>SMNLIPTVIETTNRGERAYDIYSRLLKDRIIMLGSQIDDNVANSIVSQLLFLQAQDSEKDIYLYINSPGGSVTAGFAIYDTIQHIKPDVQTICIGMAASMGSFLLAAGAKGKRFALPNAEVMIHQPLGGAQGQATEIEIAANHILKTREKLNRILSERTGQSI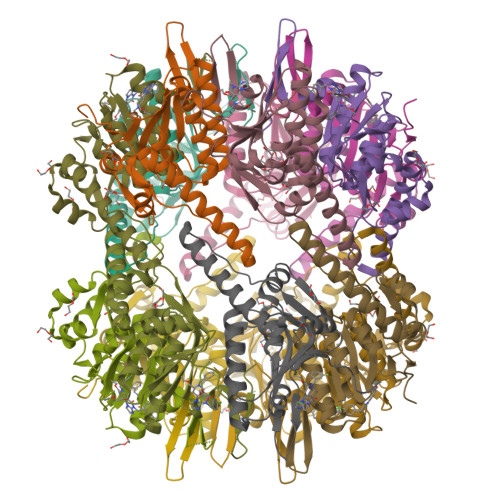EKIQKDTDRDNFLTAEEAKEYGLIDEVMVPETK[7x]> GPGAPDEV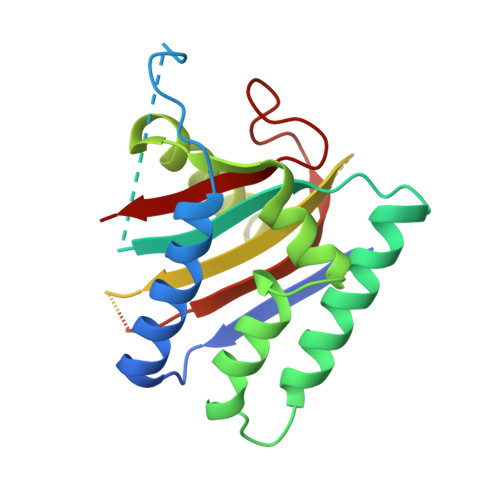IDEEVNIEFEAYSLSDNDYDGIKKLLQQLFLKAPVNTAELTDLLIQQNHIGSVIKQTDVSEDSNDDMDEDEVFGFISLLNLTERKGTQCVEQIQELVLRFCEKNCEKSMVEQLDKFLNDTTKPVGLLLSERFINVPPQIALPMYQQLQKELAGAHRTNKPCGKCYFYLLISKTFVEAGKNNSKKKPSNKKKAALMFANAEEEFFYEEQGKPEVLGGPDTRRGLEPVPIQHNGGSRGQVTALVSLKAGLIQSRSTLSDFQGTFMTVGIALS>GMSLANQIDQFLGTIMQFAENKHEILLGKSESDVKLTSTQEHILMLLAEQISTNAKIAEKLKISPAAVTKALKKLQEQELIKSSRATNDERVVLWSLTE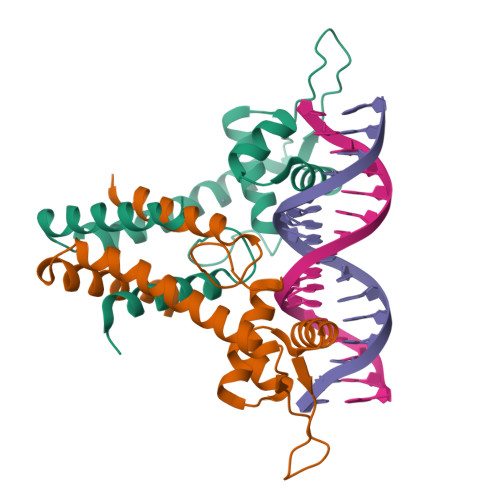KAVPVAKEHATHHEKTLSTYQELGNKFTDEEQEVISKFLSALTEEFQ[8x]>AGDIEVTGDSCNNYMLTYNKVENMTPRDLGACIDCSARHINAQVAKSHNIALIWNVKDFMSLSEQLRKQI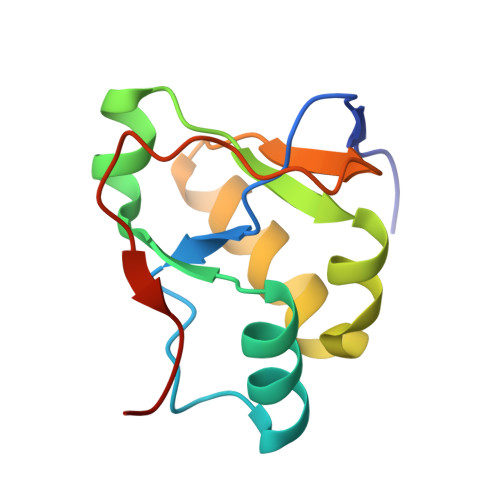RSAAKKNNLPFKLTCATTRQVVNVVTTKIALKGG[4x]>SNDASFNVETFNKTNLILQGDATVSSEGHLLLTNVKGNEEDSMGRAFYSAPIQINDRTIDNLASFSTNFTFRINAKNIENSAYGLAFALVPVGSRPKLKGRYLGLFNTTNYDRDAHTVAVVFDTVSNRIEIDVNSIRPIATESCNFGHNNGEKAEVRITYD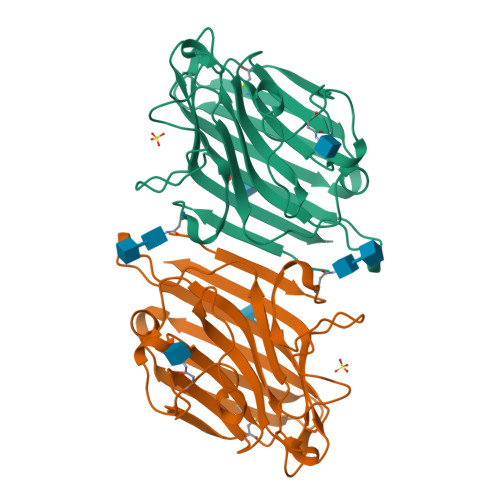SPKNDLRVSLLYPSSEEKCHVSATVPLEKEVEDWVSVGFSATSGSKKETTETHNVLSWSFSSNFI[2x]>[4x]DISKLISRGTFDQMLKHRND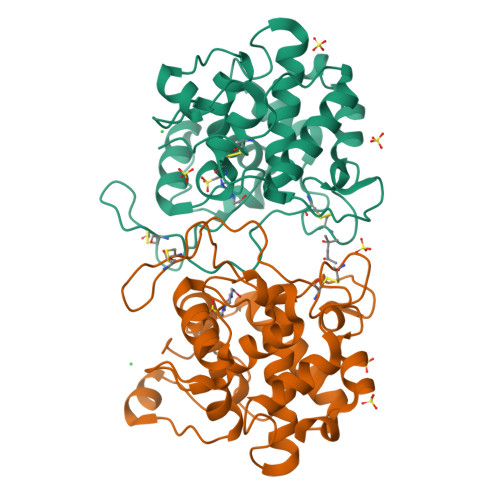GACPAKGFYTYDAFIAAAKAFPGFGTTGDDATRKREIAAFLGQTSHETTGGWASAPDGPYSWGYCFLREKNPSSSYCSPSPTYPCAAGKQYYGRGPIQLSWNYNYGQCGKAIGVDLLNNPDLVATDPVISFKTALWFWMTPQSPKPSCHNVITGIWKPSAADQSAGRVAGYGATTNIINGGLECGQGWKAQVEDRIGFYKRYCDIFKVGYGNNLDCYNQRPFGSG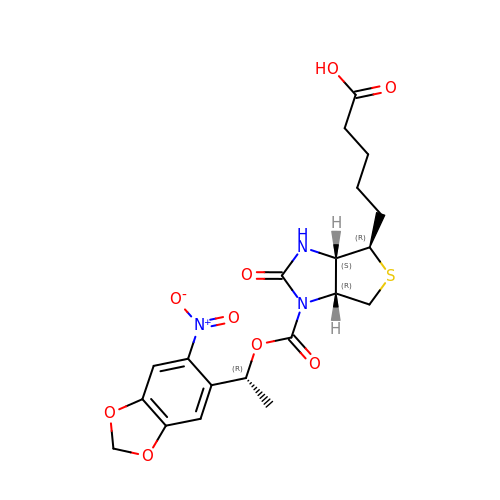5-[(3aS,4R,6aR)-1-{[(1R)-1-(6-nitro-1,3-benzodioxol-5-yl)ethoxy]carbonyl}-2-oxohexahydro-1H-thieno[3,4-d]imidazol-4-yl]pentanoic acid | C20 H23 N3 O9 S | MVOCLTWEOIJKEV-JTWAPGJUSA-N> MPSEKEILDALSKVYSEQVIQADDYFRQAIFELASQLEKEGMSSLLATKIDSLINQYILTHQFDAPKSIFDLSRLVKTKASHYKGTAISAIMLGSFLSGGPK

In order to neutralize the toxic effect of the peptide on the "producing" cell the genes encoding bacteriocins are generally co-transcribed with a cognate immunity protein. These small proteins (typically 88-115 amino acids) interact very tightly with a specific bacteriocin or pair of bacteriocins and protect the "producing" microbe from the toxic effect of its own bacteriocin. Sp-PIP belongs to a large family of putative bacteriocin immunity proteins. A combined structural, genomic and proteomic analyses has allowed the identification and in silico characterization of a new putative immunity protein from S. pyogenes.

Here we present the first structure of the protein from locus Spy_2152 (gene names taken from S. pyogenes M1 GAS), named pyogenecin immunity protein Sp-PIP, determined at 2.15 Å resolution. The crystal structure of Sp-PIP was solved by the single wavelength anomalous diffraction (SAD) method using selenomethionine (SeMet)-substituted protein. The crystal asymmetric unit contains 78 (out of the 102) well ordered residues and 74 water molecules. The first methionine and the 23 C-terminal residues are disordered and cannot be identified in the electron density maps. The four long helices (H1, residues 3-16; H3, 23-41; H4, 43-61; H5, 66-79) pack tightly together around a well-defined hydrophobic core. One additional short helix (H2, residues 17-22) connects helices H1 and H3. In the structure, the N- and C-termini are very close together (7 Å). Overall, the protein is slightly acidic (calculated pI = 6.06) with two large acidic patches near each end of the bundle and one large positively charged patch near the N- and C-termini. The structural comparison results suggest that Sp-PIP is most closely related to Imb2, from subgroup C. These results suggest that Sp-PIP is highly likely to function as a bacteriocin immunity protein with similarities to proteins from group C.> AD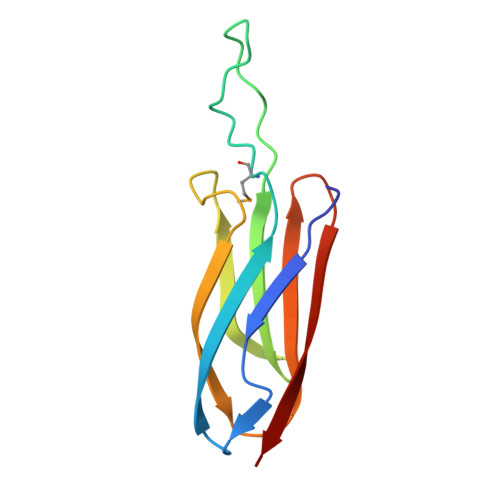DAKPRVKVPSSAKAGETVTVKALISHKMESGQRKDADGKLIPRSIINRFTCELNGVNVVDVAIDPAVSTNPYFEFDAKVDAAGEFKFTWYDDDGSVYEDVKPIAVA>AIAMTHPDISVDVLVIGAGPTGLGAAKRLNQIDGPSWMIVDSNETPGGLASTDVTPEGFLYDVGGHVIASHYKYFDDCLDEALPKEDDWYTHQRISYVRCQGQWVPYPFQNNISMLPKEEQVKCIDGMIDAALEARVANTKPKTFDEWIVRMMGTGIADLFMRPYNFKVWAVPTTKMQCAWLGERVAAPNLKAVTTNVILGKTAGNWGPNATFRFPARGGTGGIWIAVANTLPKEKTRFGEKGKVTKVNANNKTVTLQDGTTIGYKKLVSTMAVDFLAEAMNDQELVGLTKQLFYSSTHVIGVGVRGSRPERIGDKCWLYFPEDNCPFYRATIFSNYSPYNQPEASAALPTMQLADGSRPQSTEAKEGPYWSIMLEVSESSMKPVNQETILADCIQGLVNTEMLKPTDEIVSTYHRRFDHGYPTPTLEREGTLTQILPKLQDKDIWSRGRFGS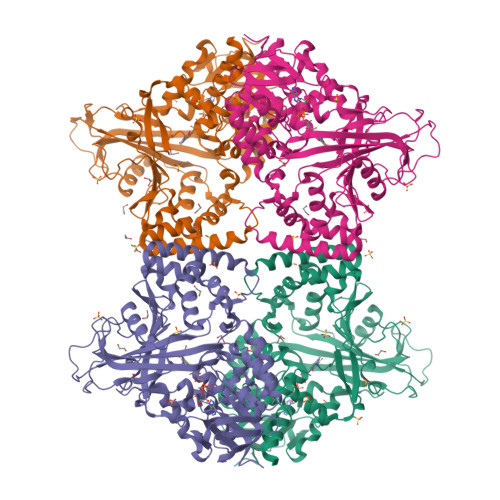WRYEVGNQDHSFMLGVEAVDNIVNGAVELTLNYPDFVNGRQNTERRLVDGAQVFAKSKAQ[4x]(2S,3R)-2-hexyl-3-hydroxynonanoic acid | C15 H30 O3 | 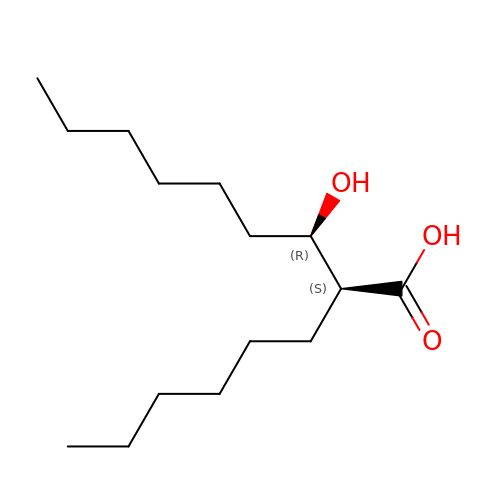PYEZBVJKCMJWAK-UONOGXRCSA-N> MAATAAEAVASGSGEPREEAGALGPAWDESQLRSYSFPTRPIPRLSQSDPRAEELIENEEPVVLTDTNLVYPALKWDLEYLQENIGNGDFSVYSASTHKFLYYDEKKMANFQNFKPRSNREEMKFHEFVEKLQDIQQRGGEERLYLQQTLNDTVGRKIVMDFLGFNWNWINKQQGKRGWGQLTSNLLLIGMEGNVTPAHYDEQQNFFAQIKGYKRCILFPPDQFECLYPYPVHHPCDRQSQVDFDNPDYERFPNFQNVVGYETVVGPGDVLYIPMYWWHHIESLLNGGITITVNFWYKGAPTPKRIEYPLKAHQKVAIMRNIEKMLGEALGNPQEVGPLLNTMIKGRYN;> NLEVAEYLLQHGADVNAQDK

2-Oxoglutarate (2OG) and Fe(II)-dependent oxygenases couple substrate oxidation with 2OG decarboxylation to give succinate and CO2; they have important functions in human biology, e.g., in hypoxia signaling, extracellular matrix biosynthesis, lipid metabolism, and DNA/RNA damage repair. The human 2OG oxygenases studied, factor inhibiting hypoxia-inducible transcription factor HIF-α (FIH) and aspartate/asparagine-β-hydroxylase (AspH), catalyze C3 hydroxylations of Asp/Asn-residues. Like AspH, human factor inhibiting the hypoxia-inducible transcription factor HIF-α (FIH) catalyzes the post-translational oxidation of Asp- and Asn-residues in a 2OG-dependent manner, however, to give the β-threo hydroxylated product. FIH was initially identified as catalyzing hydroxylation of an Asn-residue in the C-terminal transactivation domain of HIF-α isoforms (Asn803 in HIF-1α), a reaction that suppresses HIF-mediated transcription.

The nature of the FIH substrate does not seem to influence the conformation of 1, as revealed by co-crystallization with a fragment of the ankyrin repeat-containing validated human FIH substrate tankyrase-262 (FIH:1:TNKS2691–710; 2.01 Å resolution). High levels of FIH substrate hydroxylation were observed for 3-methyl-2OG and 4-methyl-2OG, both of which are natural products, regardless of the substrate, indicating that these 2OG derivatives can efficiently replace 2OG (entries 2 and 13). NMR studies reveal that FIH converts 1 and 12 into 2-methylsuccinate with a similar efficiency to which it converts 2OG into succinate. Notably, 3-methyl-2OG is an efficient cosubstrate for both FIH and AspH (entry 2), whereas its isomer 4-methyl-2OG is apparently more efficient in maintaining FIH compared with AspH activity (entry 13). The FIH Kmapp-value for 4-methyl-2OG is similar to that of 2OG, indicating a similar affinity; by contrast, the FIH Kmapp-value for 1, the 3-methyl regioisomer of 12, is higher. Although the C3/C4-alkyl 2OG derivatives were used as racemic mixtures, the crystallographic analyses reveal that, at least predominantly, the (S)-enantiomers of the 2OG derivatives bind to FIH, potentially owing to their ability to engage in more efficient hydrophobic interactions with the hydrophobic Leu186 and Leu188 sidechains. The observation that the conformations of C3- and C4-alkyl 2OG derivatives are very similar to that of 2OG in complex with FIH is in agreement with their similar Kmapp-values. The increase in length of the 2OG C3/C4-substituent from methyl via ethyl to propyl appears to correlate with enhanced FIH inhibition. Thus, although the C3/C4 methyl-substituted 2OG derivatives 1 and 12 do not inhibit FIH (entries 2 and 7), 3-propyl-2OG inhibits FIH efficiently (IC50 ~2.7 μM; Table 3, entry 4).The Mycobacterium tuberculosis (Mtb) proteasome system selectively degrades damaged or misfolded proteins and is crucial for the pathogen’s survival within the host. Mtb 20S core particle features homoheptameric rings in a conserved α7-β7-β7-α7 configuration. These rings assemble to form three interconnected compartments: two antechambers formed by α7-β7 and a central degradation chamber. Stacked β-rings enclose the degradation chamber where active sites containing the catalytic triad of βT1, βD17, and βK33 proteolyze substrates.

The fits for the 20SOG profile yielded an increased Hill coefficient of 2.3 (95% C.I. 1.9–2.7), a decreased K0.5 of 39.1 μM (95% C.I. 35.2–43.5), and unchanged Vmax of 3.4 μM s−1 (95% C.I. 3.1–3.7) as compared to 20SWT. The shift in the Hill coefficient and K0.5 values between the 20SWT and 20SOG variants points to increased cooperative interactions when the gating residues are removed. As anticipated, 20SOG successfully degraded LF2, notably with a sigmoidal concentration-dependence curve. Fitting this activity profile to the Hill model yielded a Hill coefficient of 2.0 (95% C.I. 1.7–2.3), a Vmax of 1.1 μM s−1 (95% C.I. 1.0–1.1) and a K0.5 of 8.0 μM (95% C.I. 7.1–8.9). All variants except for 20SOG display this motion, likely due to the absence of the gating residues (α2-6). Finally, analysis of the differential deuterium uptake of the 20SOG variant relative to 20SWT revealed propagation of conformational changes in the opposite direction: from the α-subunit gating residues towards the β-subunit. As expected, the structural elements immediately following the deletion site in the 20SOG variant (residues α13-33) had increased deuterium uptake relative to 20SWT. These differences, however, extended throughout the α-subunit and into the β-subunit. We measured elevated deuterium uptake in α-peptides proximal to the α-β interface, in those containing βD17 and βK33 of the catalytic triad, and in peptides from the switch helices I and II. As in previous work, stable interaction and effective degradation of pupylated substrates by Mtb Mpa-20S were only achieved in vitro with the 20SOG variant lacking the first seven residues of the α-subunits.

>[14x]MISPEQAMRERSELARKGIARAKSVVALAYAGGVLFVAENPSRSLQKISELYDRVGFAAAGKFNEFDNLRRGGIQFADTRGYAYDRRDVTGRQLANVYAQTLGTIFTEQAKPYEVELCVAEVAHYGETKRPELYRITYDGSIADEPHFVVMGGTTEPIANALKESYAENASLTDALRIAVAALRAGSADTSGGDQPTLGVASLEVAVLDANRPRRAFRRITGSALQALLVDQESPQSDGESSG;>TTIVALKYPGGVVMAGDRRSTQGNMISGRDVRKVYITDDYTATGIAGTAAVAVEFARLYAVELEHYEKLEGVPLTFAGKINRLAIMVRGNLAAAMQGLLALPLLAGYDIHASDPQSAGRIVSFDAAGGWNIEEEGYQAVGSGSLFAKSSMKKLYSQVTDGDSGLRVAVEALYDAADDDSATGGPDLVRGIFPTAVIIDADGAVDVPESRIAELARAIIESRSGADTFGSDGGEK[14x]>[2x]MKANKYLIFILGALGGLLYGYDNGV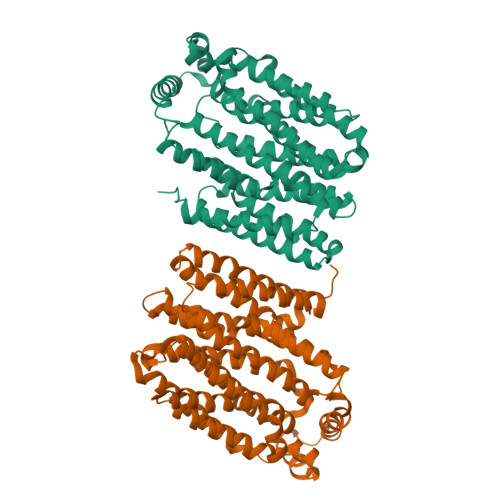ISGALLFIHKDIPLNSTTEGIVVSSMLIGAIVGAGSSGPLADKLGRRRLVMLIAIVFIIGALILAASTNLALLIIGRLIIGLAVGGSMSTVPVYLSEMAPTEYRGSLGSLNQLMITIGILAAYLVNYAFADIEGWRWMLGLAVVPSVILLVGIYFMPESPRWLLENRNEEAARQVMKITYDDSEIDKELKEMKEINAISESTWTVIKSPWLGRILIVGCIFAIFQQFIGINAVIFYSSSIFAKAGLGEAASILGSVGIGTINVLVTIVAIFVVDKIDRKKLLVGGNIGMIASLLIMAILIWTIGIASSAWIIIVCLSLFIVFFGISWGPVLWVMLPELFPMRARGAATGISALVLNIGTLIVSLFFPILSDALSTEWVFLIFAFIGVLAMIFVIKFLPETRGRSLEEIEYELRERTGARTE>EDGYDMWLRYQPIADQTLLKTYQKQIRHLHVAGDSPTINAAAAELQRGLSGLLNKPIVARDEKLKDYSLVIGTPDNSPLIASLNLGERLQALGAEGYLLEQTRINKRHVVIVAANSDVGVLYGSFHLLRLIQTQHALEKLSLSSAPRLQHRVVNHWDNLNRVVERGYAGLSLWDWGSLPNYLAPRYTDYARINASLGINGTVINNVNADPRVLSDQFLQKIAALADAFRPYGIKMYLSINFNSPRAFGDVDTADPLDPRVQQWWKTRAQKIYSYIPDFGGFLVKADSAGQPGPQGYGRDHAEGANMLAAALKPFGGVVFWRAFVYHPDIEDRFRGAYDEFMPLDGKFADNVILQIKNGPIDFQPREPFSALFAGMSRTNMMMEFQITQEYFGFATHLAYQGPLFEESLKTETHARGEGSTIGNILEGKVFKTRHTGMAGVINPGTDRNWTGHPFVQSSWYAFGRMAWDHQISAATAADEWLRMTFSNQPAFIEPVKQMMLVSREAGVNYRSPLGLTHLYSQGDHYGPAPWTDDLPRADWTAVYYHRASKTGIGFNRTKTGSNALAQYPEPIAKAWGDLNSVPEDLILWFHHLSWDHRMQSGRNLWQELVHKYYQGVEQVRAMQRTWDQQEAYVDAARFAQVKALLQVQEREAVRWRNSCVLYFQSVAGRPIPANYEQPEHDLE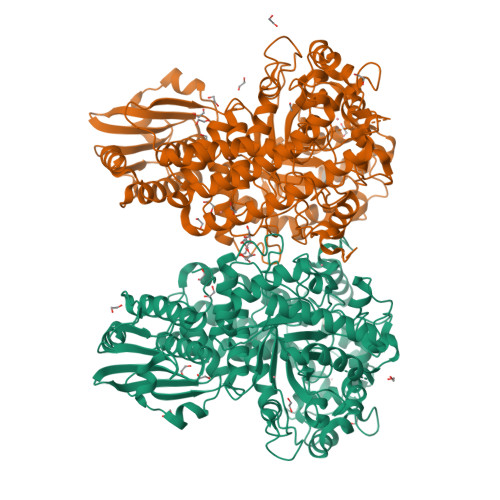YYKMLARTTYVPEPWHPASSSRVLK[2x]> SVDMALGDLMVSRFSQSSVSLVSNHRYDEDCVSSHDDGDSRRKDSEAKSSSSYGNGTTEGAATATSMAYLPQTIVLCELRHDASEASAPLGTSEIVLVPKWRLKERMKTGCVALVLCLNITVDPPDVIKISPCARIEAWIDPFSMAPPKALETIGKNLSTQYERWQPRARYKVQLDPTVDEVRKLCLTCRKYAKTERVLFHYNGHGVPKPTANGEIWVFNKSYTQYIPLPISELDSWLKTPSIYVFDCSAARMILNAFAELHDWGSSGSSGSSRDCILLAACDVHETLPQSVEFPADVFTSCLTTPIKMALKWFCRRSLLKEIIDESLIDRIPGRQNDRKTLLGELNWIFTAVTDTIAWNVLPHELFQRLFRQDLLVASLFRNFLLAERIMRSANCNPISHPMLPPTHQHHMWDAWDMAAEICLSQLPQLVLDPSTEFQPSPFFTEQLTAFEVWLDHGSEHKKPPEQLPIVLQVLLSQCHRFRALVLLGRFLDMGSWAVDLALSVGIFPYVLKLLQTTTNELRQILVFIWTKILALDKSCQIDLVKDGGHTYFIRFLDSSGAFPEQRAMAAFVLAVIVDGHRRGQEACL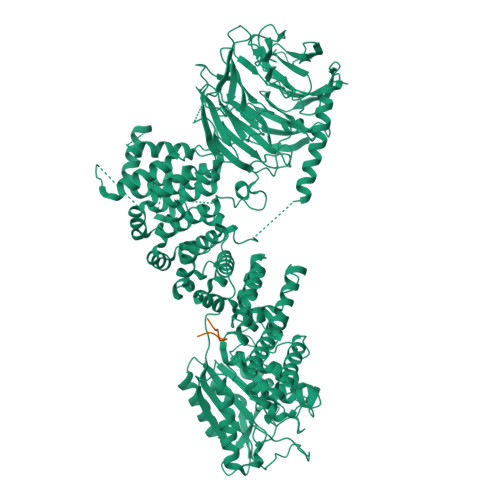EANLIGVCLGHLEASRPSDPQPEPLFLQWLCLCLGKLWEDFMEAQIMGREANAFEKLAPLLSEPQPEVRAAAVFALGTLLDIGFDSNKSVVEDEFDDDEKIRAEDAIIKSLLDVVSDGSPLVRAEVAVALARFAFGHKQHLKLAAASYWKPQSSSLLTSLPSIAKFHDPGSATIVSLHMSPLTRASTDSQPVARESRISSSPLGSSGLMQGSPLSDDSSLHSDSGMMHDSVSNGAVHQPRLLDNAVYSQCVRAMFALAKDPSPRIASLGRRVLSIIGIEQVVAKPSKPTGRPGEAADSGLADPLLGASGSERSLLPLSTIYGWSCGHFSKPLLGGADASQEIAAKREEKEKFALEHIAKCQHSSISKLNNNPIANWDTRFETGTKTALLHPFSPIVVAADENERIRVWNYEEATLLNGFDNHDFPDKGISKLCLINELDDSLLLVASCDGSVRIWKNYATKGKQKLVTGFSSIQGHKPGARDLNAVVDWQQQSGYLYASGETSTVTLWDLEKEQLVRSVPSESECGVTALSASQVHGGQLAAGFADGSLRLYDVRSPEPLVCATRPHQKVERVVGLSFQPGLDPAKVVSASQAGDIQFLDLRTTRDTYLTIDAHRGSLTALAVHRHAPIIASGSAKQLIKVFSLQGEQLGIIRYYPSFMAQKIGSVSCLTFHPYQVLLAAGAADSFVSIYTHDNSQAR;> RNSPEDKRAGGEESQFEMDI>[2x]GSHMAHQPSDTIAGLYEAFNSGDLETLRELIAPDAVIHLPGTAGDAEHPPGTPRDREGWLGVWQFTQAFFPDMTATVQDIVQTGDLVATRCVARGTHSGRPFEMTML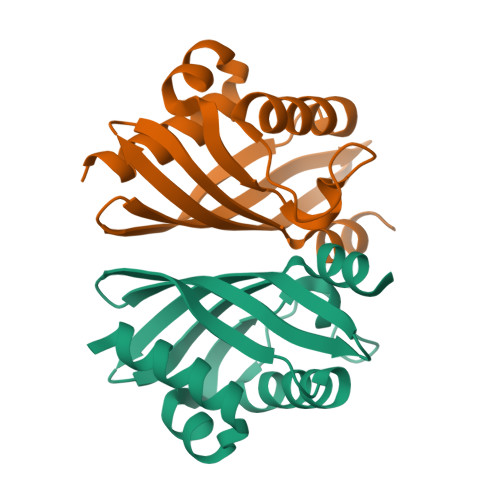NMSRVRDGRIVEHWTISDNVTMLAQLGVKASL>[2x]MVITLPKLKYALNALSPHISEETLNFHYNKHHAGYVNKLNTLIKDTPFAEKSLLDIVKESSGAIFNNAAQIWNHTFYWDSMGPDCGGEPHGEIKEKIQE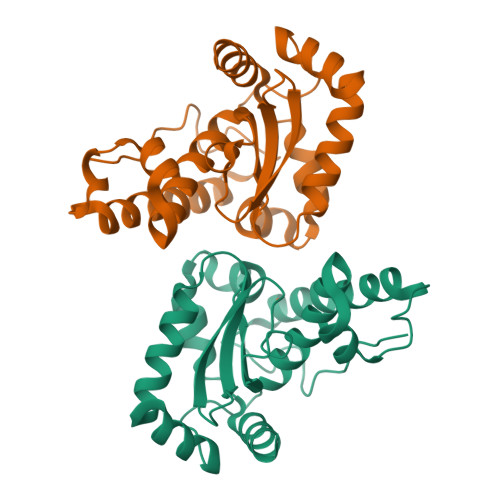DFGSFNNFKEQFSNILCGHFGSGWGWLALNNNNKLVILQTHDAGNPIKDNTGIPILTCDIWEHAYYIDYRNDRASYVKAWWNLVNWNFANENLKKAMQKLEHHHHHH>[2x]MVEQIKDKLGRPIRDLALSVTDRCNFRCDYCMPKEVFGDDFVFLPKNELLTFDEMARIAKVYAELGVKKIRITGGEPLMRRDLDVLIAKLNQIDGIEDIGLTTNGLLLKKHGQKLYDAGLRRINVSLDAIDDTLFQSINNRNIKATTILE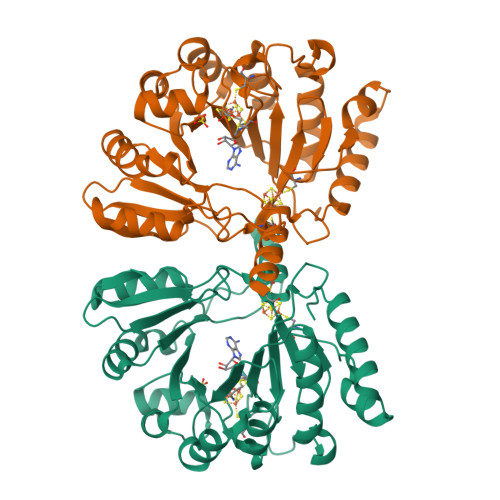QIDYATSIGLNVKVNVVIQKGINDDQIIPMLEYFKDKHIEIRFIEFMDVGNDNGWDFSKVVTKDEMLTMIEQHFEIDPVEPKYFGEVAKYYRHKDNGVQFGLITSVSQSFCSTCTAAALSSDGKFYGCLFATVDGFNVKAFIRSGVTDEELKEQFKALWQIRDDRYSDERTAQTVANRQRKKINMNYIGG>MMNPLIIKLGG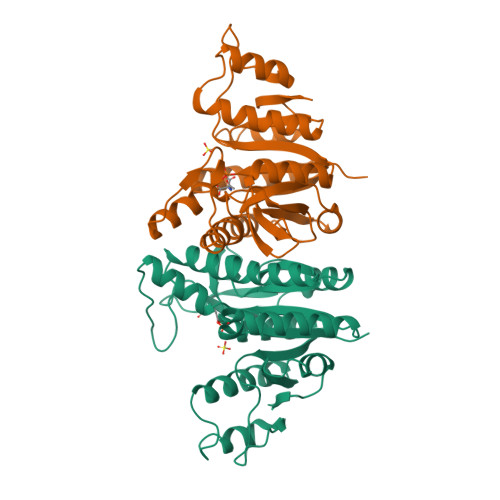VLLDSEEALERLFSALVNYRESHQRPLVIVHGGGCVVDELMKGLNLPVKKKNGLRVTPADQIDIITGALAGTANKTLLAWAKKHQIAAVGLFLGDGDSVKVTQLDEELGHVGLAQPGSPKLINSLLENGYLPVVSSIGVTDEGQLMNVNADQAATALAATLGADLILLSDVSGILDGKGQRIAEMTAAKAEQLIEQGIITDGMIVKVNAALDAARTLGRPVDIASWRHAEQLPALFNGMPMGTRILA[2x]> MHHHHHHENLYFQGTKDLN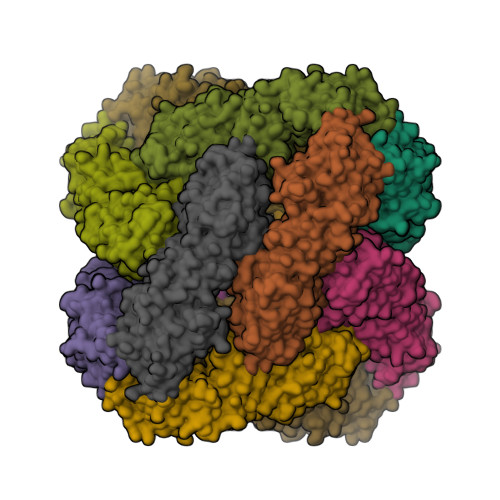TLVSELPEIYQTIFGHPEWDGDAARDCNQRLDLITEQYDNLSRALGRPLNVLDLGCAQGFFSLSLASKGATIVGIDFQQENINVCRALAEENPDFAAEFRVGRIEEVIAALEEGEFDLAIGLSVFHHIVHLHGIDEVKRLLSRLADVTQAVILELAVKEEPFYWGVSQPDDPRELIEQCAFYRLIGEFDTHLSPVPRPMYLVSNHRVLINDFNQPFQHWQNQPYAGAGLAHKRSRRYFFGEDYVCKFFYYDMPHGILTAEESQRNKYELHNEIKFLTQPPAGFDAPAVLAHGENAQSGWLVMEKLPGRLLSDMLAAGEEIDREKILGSLLRSLAALEKQGFWHDDVRPWNVMVDARQHARLIDFGSIVTTPQDCSWPTNLVQSFFVFVNELFAENKSWNGFWRSAPVHPFNLPQPWSNWLYAVWQEPVERWNFVLLLALFEKKAKLPSAEQQRGATEQWIIAQETVLLELQSRVRNESAGSEALRGQIHTLEQQMAQLQSAQDAFVEKAQQPVEVSHELTWLGENMEQLAALLQTAQAHAQADVQPELPP>[2x]MEVLFEAKVGDITLKLAQGDITQYPAKAIVNAANKRLEHGGGVAYAIAKACAGDAGLYTEISKKA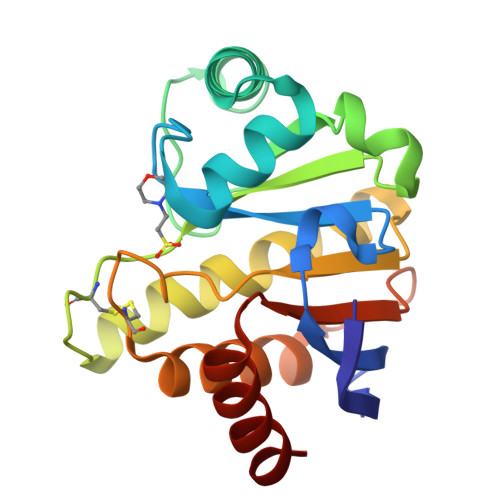MREQFGRDYIDHGEVVVTPAMNLEERGIKYVFHTVGPICSGMWSEELKEKLYKAFLGPLEKAEEMGVESIAFPAVSAGIYGCDLEKVVETFLEAVKNFKGSAVKEVALVIYDRKSAEVALKVFERSL>SSQSSKIFKNCVIYINGYTKPGRLQLHEMIVLHGGKFLHYLSSKKTVTHIVASNLPLKKRIEFANYKVVSPDWIVD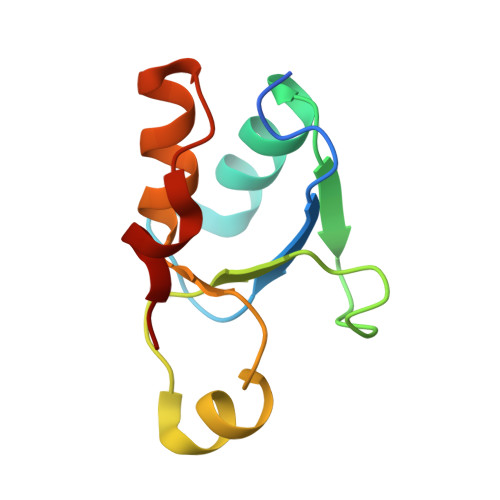SVKEARLLPWQNYSLT[2x]>[2x]QDGKTTFEKEGGGGRGPRILENMHESSCKYEKNWPICVDDDWGTKCPSCCRMQGIIDDTDQNYSQRIDNIRQQLADSQNKYKTSNRVIVETINILKPGLEGAQQLDENYGHVSTELRRRIVTLKQRVA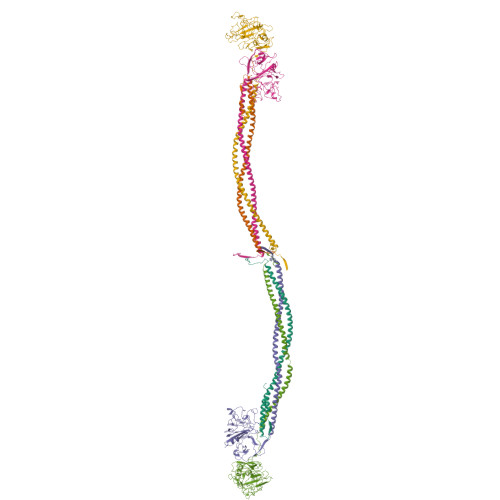TQVNRIKALQNSIQEQVVEMKRLEVDIDIKIRACKGSCARSFDYQVDKEGYDNIQKHLTQASSIDMHPDFQTTTLSTLKMRPLKDSNVPEHFKLKPSPEMQAMSAFNNIKQMQVVLERPETDHVAEARGDSSPSHTGKLITSSHRRESPSLVDKTSSASSVHRCTRTVTKKVISGPDGPREEIVEKMVSSDGSDCSHLQGGREGSTYHFSGTGDFHKLDRLLPDLESFFTHDSVSTSSRHSIGSSTSSHVTGAGSSHLGTGGKDKFTDLGEEEEDDFGGLQPSGFAAGSASHSKTVLTSSSSSFNKGGSTFETKSLKTRETSEQLGGVQHDQSAEDTPDFKARSFRPAAMSTRRSYNGKGTQK;>[2x]QASVEYDNEEDSPQIDARAHRPLDKRQEAAPTLRPVAPPISGTGYQPRPPKQDKQAMKKGPIIYPDAGGCKHPLDELGVLCPTGCELQTTLLKQEKTVKPVLRDLKDRVAKFSDTSTTMYQYVNMIDNKLVKTQKQRKDNDIILSEYNTEMELHYNYIKDNLDNNIPSSLRVLRAVIDSLHKKIQKLENAIATQTDYCRSPCVASCNIPVVSGRECEDIYRKGGETSEMYIIQPDPFTTPYRVYCDMETDNGGWTLIQNRQDGSVNFGRAWDEYKRGFGNIAKSGGKKYCDTPGEYWLGNDKISQLTKIGPTKVLIEMEDWNGDKVSALYGGFTIHNEGNKYQLSVSNYKGNAGNALMEGASQLYGENRTMTIHNGMYFSTYDRDNDGWLTTDPRKQCSKEDGGGWWYNRCHAANPNGRYYWGGTYSWDMAKHGTDDGIVWMNWKGSWYSMKKMSMKIKPYFPD;>[2x]YIATRENCCILDERFGSYCPTTCGIADFFNKYRLTTDGELLEIEGLLQQATNSTGSIEYLIQHIKTIYPSEKQTLPQSIEQLTQKSKKIIEEIIRYENTILAHENTIQQLTDMHIMNSNKITQLKQKIAQLESHCQEPCKDTAEIQETTGRDCQDIANKGARKSGLYFIKPQKAKQSFLVYCEIDTYGNGWTVLQRRLDGSEDFRRNWVQYKEGFGHLSPDDTTEFWLGNEKIHLITTQSTLPYALRIELEDWSGKKGTADYAVFKVGTEEDKYRLTYAYFIGGERGDAFDGFNFGDDPSDKSYTYHNGMRFSTFDNDNDNFEGNCAEQDGSGWWMNRCHAGHLNGPYYIGGVYSRDTGTNSYDNGIIWATWRDRWYSMKKTTMKIIPFNRLSIDGQQHSGGLKQVGDS> MAASWRLGCDPRLLRYLVGFPGRRSVGLVKGALGWSVSRGANWRWFHSTQWLRGDPIKILMPSLSPTMEEGNIVKWLKKEGEAVSAGDALCEIETDKAVVTLDASDDGILAKIVVEEGSKNIRLGSLIGLIVEEGEDWKHVEIPKDVGP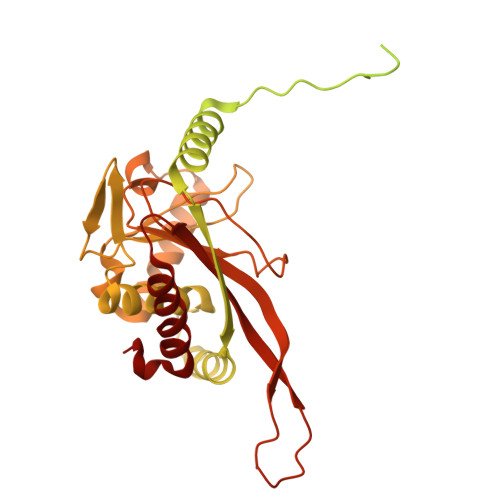PPPVSKPSEPRPSPEPQISIPVKKEHIPGTLRFRLSPAARNILEKHSLDASQGTATGPRGIFTKEDALKLVQLKQTGKITESRPTPAPTATPTAPSPLQATAGPSYPRPVIPPVSTPGQPNAVGTFTEIPASNIRRVIAKRLTESKSTVPHAYATADCDLGAVLKVRQDLVKDDIKVSVNDFIIKAAAVTLKQMPDVNVSWDGEGPKQLPFIDISVAVATDKGLLTPIIKDAAAKGIQEIADSVKALSKKARDGKLLPEEYQGGSFSISNLGMFGIDEFTAVINPPQACILAVGRFRPVLKLTEDEEGNAKLQQRQLITVTMSSDSRVVDDELATRFLKSFKANLENPIRLA D-Glyceraldehyde | C3 H6 O3 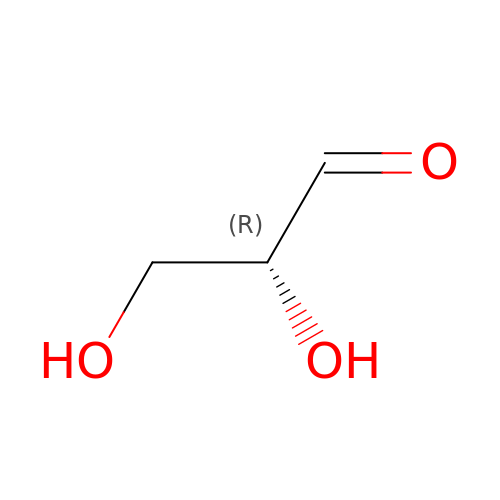| MNQZXJOMYWMBOU-VKHMYHEASA-N> MSRFSVLSFLILAIFLGGSIVKGDVSFRLSGADPRSYGMFIKDLRNALPFREKVYNIPLLLPSVSGAGRYLLMHLFNYDGKTITVAVDVTNVYIMGYLADTTSYFFNEPAAELASQYVFRDARRKITLPYSGNYERLQIAAGKPREKIPIGLPALDSAISTLLHYDSTAAAGALLVLIQTTAEAARFKYIEQQIQERAYRDEVPSLATISLENSWSGLSKQIQLAQGNNGIFRTPIVLVDNKGNRVQITNVTSKVVTSN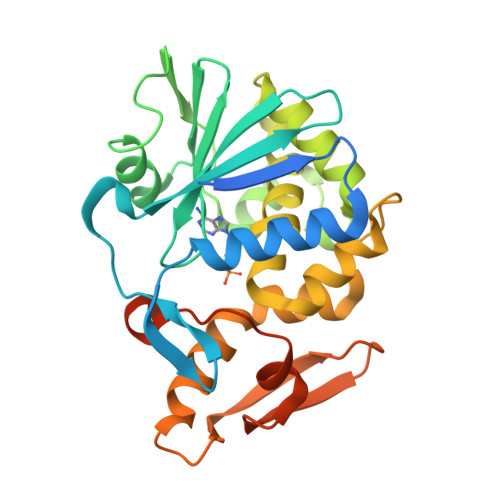IQLLLNTRNIAEGDNGDVSTTHGFSSY> APTKRKGECPGAAPKKPKEPVQVPKLLIKGGVEVLEVKTGVDAITEVECFLNPEMGDPDENLRGFSLKLSAENDFSSDSPERKMLPCYSTARIPLPNLNEDLTCGNLLMWEAVTVQTEVIGITSMLNLHAGSQKVHEHGGGKPIQGSNF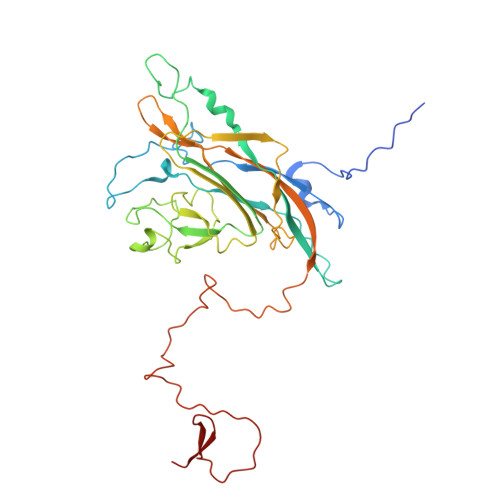HFFAVGGDPLEMQGVLMNYRTKYPDGTITPKNPTAQSQVMNTDHKAYLDKNNAYPVECWVPDPSRNENTRYFGTFTGGENVPPVLHVTNTATTVLLDEQGVGPLCKADSLYVSAADICGLFTNSSGTQQWRGLARYFKIRLRKRSVKNPYPISFLLSDLINRRTQRVDGQPMYGMESQVEEVRVFDGTERLPGDPDMIRYIDKQGQLQTKML> MDTTVPTFSLAELQQGLHQDEFRRCLRDKGLFYLTDCGLTDTELKSAKDIVIDFFEHGSEAEKRAVTSPVPTMRRGFTGLESESTAQITNTGSYSDYSMCYSMGTADNLFPSGDFERIWTQYFDRQYTASRAVAREVLRATGTEPDGGVEAFLDCEPLLRFRYFPQVPEHRSAEEQPLRMAPHYDLSMVTLIQQTPCANGFVSLQAEVGGAFTDLPYRPDAVLVFCGAIATLVTGGQVKAPRHHVAAPRRDQIAGSSRTSSVFFLRPNADFTFS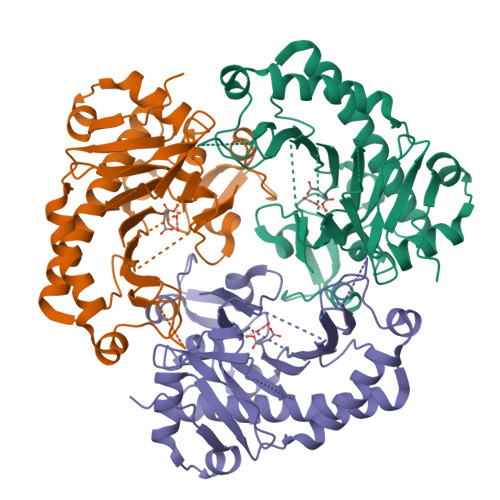VPLARECGFDVSLDGETATFQDWIGGNYVNIRRA> ARQREIEMNRQQRFFRIPFIRPADQYKDPQSKKKG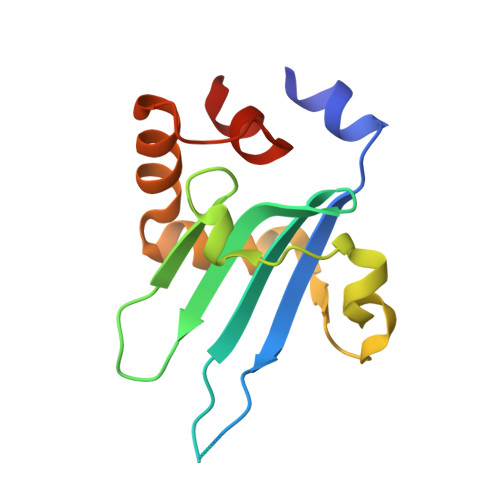WWYAHFDGPWIARQMELHPDKPPILLVAGKDDMEMCELNLEETGLTRKRGAEILPRQFEEIWERCGGIQYLQNAIESRQARPTYATAMLQSLLK> EAQQKTIEAITKAINYMAKRRIGALLTIERDTGMGDYIETGIPLNAKVSSELLINIFIPNTPLHDGAVIMKNNEIAAAACYLPLSESPFISKELGTRHRAAVGISEVTDSLTIIVS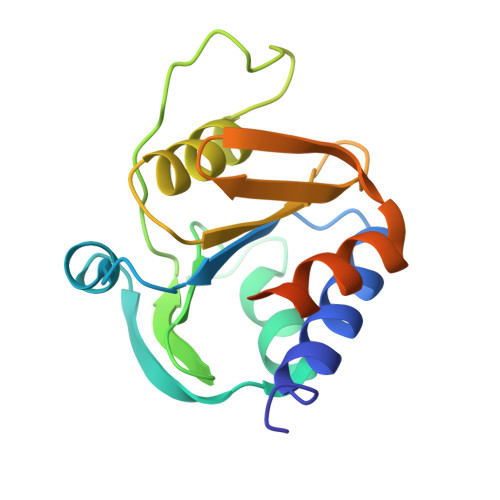EETGGVSVAKNGDLHRELTEEALKEMLEAEFKKNTRDTSSNRWYWRGKKNG1-KETO,2-HYDROXY,4-NITROBENZENE, 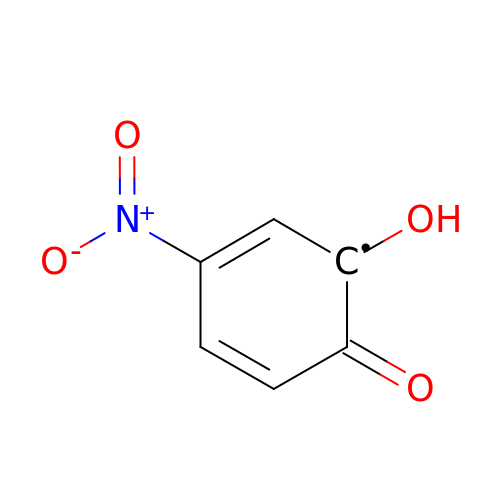1 ELECTRON OXIDIZED | C6 H4 N O4 | KJBVYJMPBKCQJZ-ZCFIWIBFSA-N>MAHHHHHHMSFKPKIIVCGSPAELSGVACKKIVEIIHASERTNWPLSIALSGGSTPKMLYSLLHEEHLHLLKEERALRFFFGDERLVPADAAESNYNMARQALLRDIPEDLVVPVDVGCVGKVSKVACNDAVKSADAYEKKIALLLGTQKVEGMEAEIPVFDIVLLGLGSDGHTASIFHGSQAESEMHRAVSVGFPSPTMSPKVWRVTLTPITIIHARHVILLATGKEKKCVLNGIIADTPTEVPVSRFLRNCKGD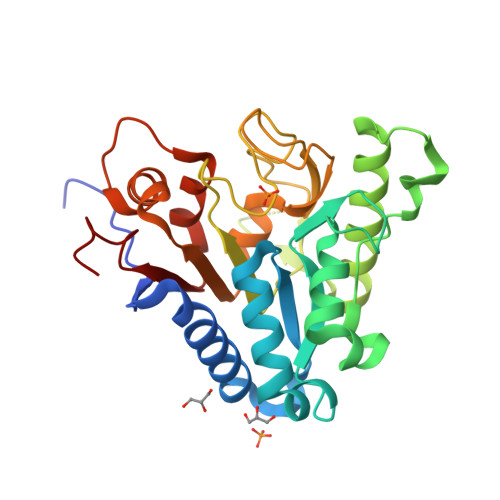VTFILDKEIAENLTC[2x]> 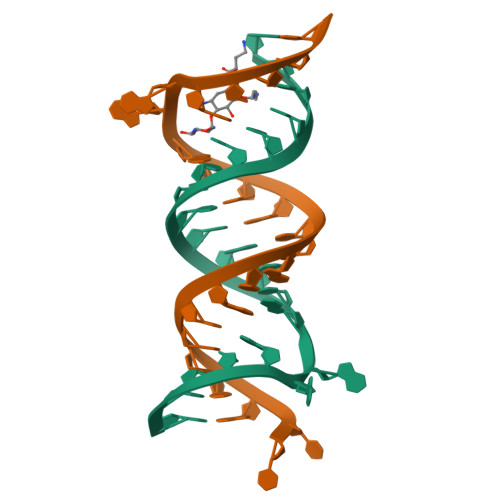GCGUCACACCGGUGAAGUCGC;> UUGCGUCACACCGGUGAAGUCGC Here, we describe the synthesis of 2′-position unmodified 5′-(R)- and 5′-(S)-C-methyl guanosine and evaluation of these nucleotides in the context of siRNA. The (R) isomer provided protection from 5′ exonuclease and the (S) isomer provided protection from 3′ exonuclease in the context of a terminally modified oligonucleotide. siRNA potency was maintained when these modifications were incorporated at the tested positions of sense and antisense strands. Structural properties of 5′-(R)-C-methyl guanosine incorporated into an RNA octamer were analysed by X-ray crystallography, and the structure explains the loss in duplex thermal stability for the (R) isomer compared with the (S) isomer. To evaluate the effect of 5′-C-methyl guanosine on thermal melting of duplexes and to analyse the effects of the 5′-C-methyl modification on the backbone geometry of RNA, we characterized self-complementary RNA octamers, 5′-CCCCXGGG-3′, where X is either 5′-(R)- or 5′-(S)-C-methyl-guanosine.

Crystals of the octamer modified with 5′-(R)-C-methyl-guanosine diffracted to 1.56-Å resolution, and the structure was phased by molecular replacement. In addition to the single RNA duplex per asymmetric crystallographic unit in the hexagonal unit cell, five Co(III) hexamine ions and 30 water molecules were included in the final model. The riboses of modified guanosines adopt the C3′-endo pucker and the 5′-C-methyl groups exhibit short intra-nucleotide 1…5 contacts to O3′ and OP1 atoms with distances of between 3.0 and 3.15 Å. The backbone torsion angles α to ζ for the modified guanosines fall into the standard sc−, ap, sc+, sc+, ap and sc− ranges that are characteristic of A-form duplexes. In the reference structure, G13 has an extended backbone as a result of a crankshaft motion around torsion angle β that flips both α and γ into the ap range. However, this is not the case with the 5′-(R)-C-methyl-modified G13. A model with an (R)-configured methyl group attached to G13 of the parent duplex (stretched backbone) reveals contacts between methyl carbon and OP2 and guanine C8 of 2.7 and 2.4 Å, respectively. Thus, it appears that short contacts with O3′ and OP1 as a consequence of an (R) isomer are unavoidable. The 5′-(R)-C-methyl interferes with hydration between adjacent phosphate groups. In contrast, the 5′-(S)-C-methyl is directed away from the hydration network around the phosphate backbone, consistent with the greater loss in duplex thermal stability previously reported for incorporation of the (R) isomer compared with the (S) isomer.

>[2x]CCCCXGGG>AMDQKQFEKIRAVFDRSGVALTLVDMSLPEQPLVLANPPFLRMTGYTEGQILGFNCRFLQRGDENAQARADIRDALKLGRELQVVLRNYRANDEPFDNLLFLHPVGGRPDAPDYFLGS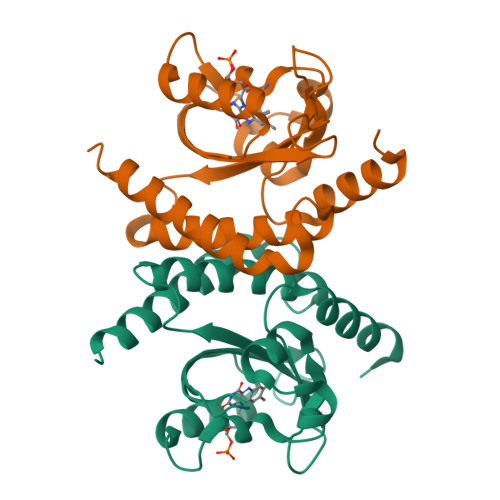QFELGRSGNSEEAAAAGHAGALTGELARIGTVAARLEMDSRRHLAQAAAALVRAWERRG[2x]>[6x]MRYRPFGSTGVAVSALTLRLADNPRLRANDWRALVFTALENGVNSFQIDGDAPELLKGAGEAFASVERHLLFLTWRLRGDAKQLGPHTLDALKRSAFEGLSLDYLDLLLINDPQSASLPMAFESGLQDLQKGRALRGLGVASRGDIDPGLLANDLVTAVSSPYNLSSGWAERHRIRQASQNNFAVIGEDFWPQALREV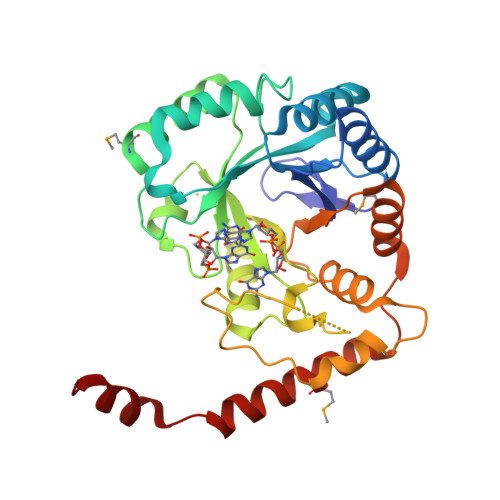VADKAPPKPSFWQRRTDPLADVGGYEFLTNTPGWSAEDICLGYALTEPSLATVRVTADNRQEIERLAAVVERDLPTGVCAQIEMARFSAQEREKAARRPKLAAALEHHHH> GS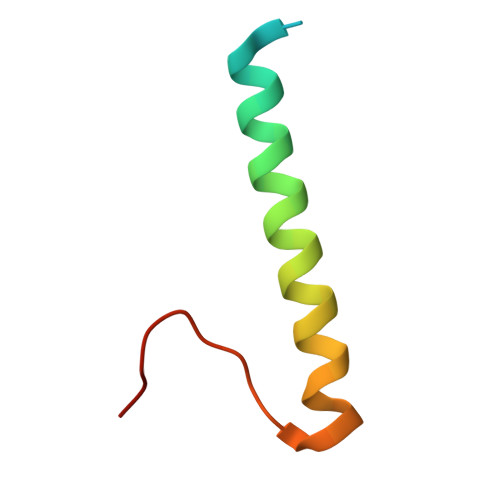HMEADTAMRDLILHQRELLKQWTEYREKIGQEMEKSMNFKIFDVQPED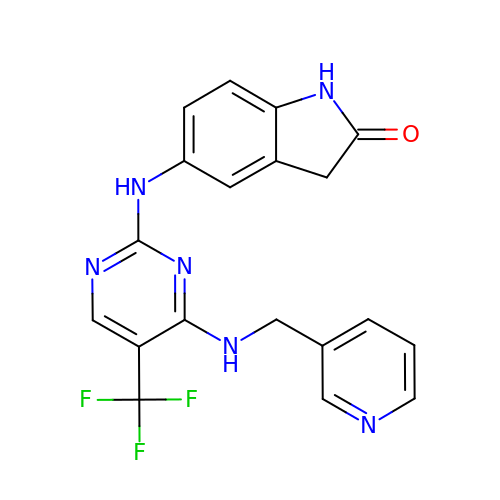5-[[4-(pyridin-3-ylmethylamino)-5-(trifluoromethyl)pyrimidin-2-yl]amino]-1,3-dihydroindol-2-one | C19 H15 F3 N6 O | HOEAQQRLTIBABU-UHFFFAOYSA-N> MRAVNWNKKEDDFSLMFWKQNIAQFWTEEEIAVSSDKNTWVQLSKEEQIAYKRVLGGLTLLDTKQGGEGMPLVLVHLENLQAKSVLAFMGAMEEVHAKSYSHIFTTLATEEEIDDIFDWVDNHPLLEKKAGIITSYYRRLLKPEVTKKELYMAMVASVFLESYLFYSGFFYPLYLAGQGKLTASGEIINLIIRDESIHGVFVGILAQQIFAELSAEEQQEVQKETQELLMELYEIEMAYTEEIYTSIGLVEDVNRFVRYNANKGLMNLGLEPKFEEEEINPIVLNGLRTDTKNHDFFSVKGNGYVKATNVEKLADDDFVFNF;> MLVAYDSMTGNVKRFIHKLNMPAVQIDEDLVIDEDFILITYTTGFGNVPERVLDFLERNNEKLKGVSASGNRNWGDMFGASADKISTKYEVPIVSKFELSGTNNDVEYFKERVREIATH

Ribonucleotide reductases (RNRs) are essential metalloenzymes that employ sophisticated radical chemistry to reduce the 2′-OH group of ribonucleotides and thereby produce deoxyribonucleotides (dNTPs), the building blocks of DNA. The class Ib R2 subunit (R2b) metal site can bind two manganese ions or two iron ions. In contrast, the di-manganese R2b form cannot react with O2 but requires a superoxide radical (O2•−) provided by NrdI, a flavoprotein which is generally encoded in the same operon as R2b (Berggren et al., 2014; Cotruvo and Stubbe, 2010; Roca et al., 2008). NrdI binds tightly to R2b in a 1:1 ratio with FMN at the protein–protein interface, forming a dimer of heterodimers.

The crystals for the first dataset were grown under aerobic conditions, yielding bright orange crystals, indicating that NrdI was fully oxidized. In BcR2bMnMn–NrdIox, the isoalloxazine moiety of FMNox is almost planar, with a butterfly bend of 0.2°. An unknown molecule is bound within 5 Å from the reactive C4a of FMN in BcR2bMnMn–NrdIox, which binds O2 to reduce it to O2•−. The molecule is 3-coordinated to Trp74 (NrdI), Ser196 (R2b), and a water (p-ox in Figure 5D, E). The exact nature of the molecule could not be determined and was thus designated as an unknown atom in the final model. The position of the density in BcR2bMnMn–NrdIox is close to the channel entrance on the R2b surface marked by Lys263, Asn267, and Ser196. In BcR2bMnMn–NrdIox, the two metal ions of R2b are refined at full occupancy and the coordination sphere is clearly defined in the electron density map. Mn1 is 4-coordinated by His96, Glu93, Asp62, and Glu195. Mn2 is 5-coordinated by His198, Glu93, Glu195, and Glu161. The protein complex used in the crystallization for the BcR2bMnMn–NrdIox dataset has not undergone any oxidation of the metal site and both manganese ions are in the Mn(II)/Mn(II) oxidation state.>MMSETAPLPSASSALE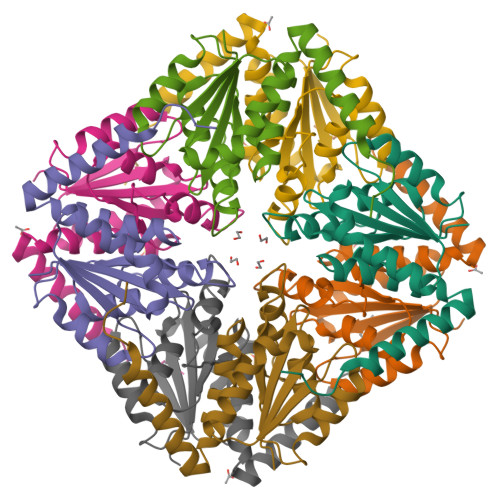DKAASAPVVGIIMGSQSDWETMRHADALLTELEIPHETLIVSANRTPDRLADYARTAAERGLNVIIAGAGGAAHLPGMCAAWTRLPVLGVPVESRALKGMDSLLSIVQMPGGVPVGTLAIGASGAKNAALLAASILALYNPALAARLETWRALQTASVPNSPITEDK[2x]CYCLOHEXANOL | C6 H12 O | 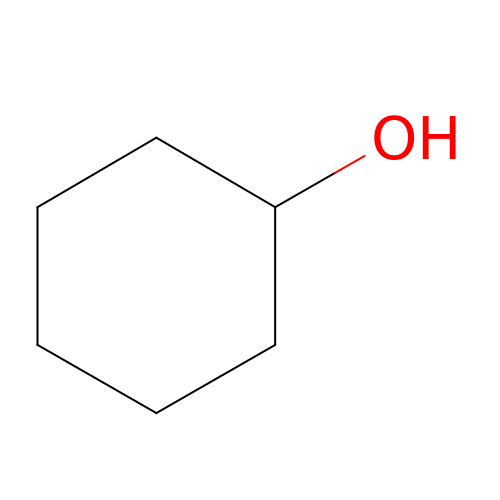HPXRVTGHNJAIIH-UHFFFAOYSA-N>[4x]GPAMEALELELEEVESQIRALVVRRSRLRERLLAVP

Instead of Gag, non-LTR retrotransposons frequently encode a distinct multidomain protein named ORF1p, which is translated from the first open reading frame (ORF1). To learn whether the esterase domain is more than a mere molecular fossil and to learn about the potential functions of esterase-encoding ORF1ps in non-LTR retrotransposition, we took a structure-based approach and characterized the ORF1p of the ZfL2-1 non-LTR retrotransposon from zebrafish, Danio rerio. We defined the boundaries of two functional domains and determined their crystal structures. We also demonstrate that the esterase is enzymatically active and binds to negatively charged liposomes. Together, these findings define a third class of ORF1p architecture and suggest that lipids may play a role in non-LTR retrotransposition.

The first structure is that of an N-terminal coiled coil domain that we show to cause a dimerization of the molecule, an assembly mode that is clearly distinct from the trimers formed by the LINE-1 ORF1p. In analytical SEC, the N-terminal construct indeed shows self-interaction and we find it to exclusively form dimers, whereas the esterase domain remains monomeric at concentrations up to 75 µM. A proteolytically stable fragment of the N-terminal construct gave crystals that contained two copies of an antiparallel homodimeric coiled coil per asymmetric unit, and the structure was refined to an Rfree of 21.5% at 1.55 Å resolution. Each α-helix comprises five heptad repeats, confining the coiled coil to the region between M15 and P47 as we would predict from the sequence. Because of the charge compensation between the highly acidic N-terminal heptads and the highly basic C-terminal heptads, we presume a preference for the antiparallel orientation also in the absence of crystal packing constraints, an arrangement that is clearly distinct from the parallel trimeric coiled coil formed by the LINE-1 ORF1p. Whereas coiled coil domains and their ability to multimerize are hence frequently present among ORF1ps, the resulting assemblies can differ significantly in terms of structure and likely do not always have a common evolutionary origin.> MKTVLIGVGQAGGKLASALQSFDRQTGFGAVLDAVAVNTAKADLQSLPVETVLIGQDRVNGHGVGGDNELGAAVMESDQTEVMSALDGRVTAEAESIFVVAGLGGGSGSGGAPVLAKALAGVYDVPVYVLGILPGADEGALYQVNAGRSLKTVAREADAVLLVDNDAFRSAGESMSEGYDAINEAIARRVGLLLAAGEATEGVGESVVDTSEVINTLRSGGIAALGYASAEASPNAEDNINAVMSTTRRAVLTGTSLPDASDADAALVVIAGEPDTIPRKGVERARRWVEDETGSMQVRGGDFPLESGRLASLVLLGGVERSERVE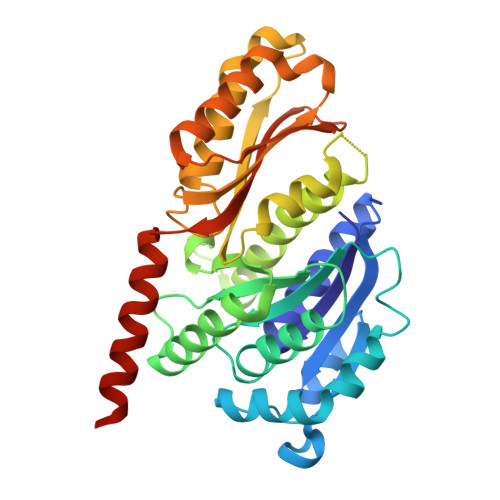SFMERAREAIDKAETEPREDPKG2-O-phosphono-alpha-L-arabinopyranose | C5 H11 O8 P | 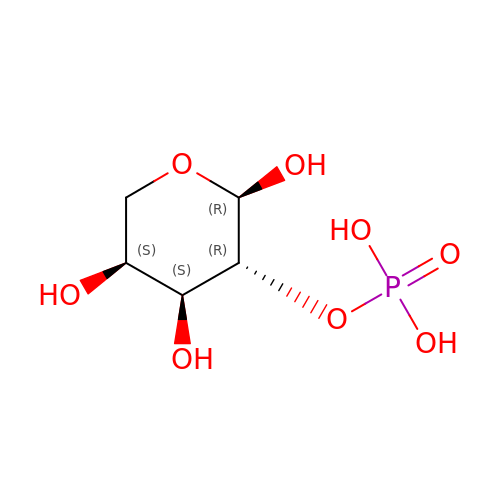QIAIUTJEZJIPSH-QMKXCQHVSA-N> SSLDDKPQFPGASAEFIDKLEFIQPNVISGIPIYRVMDRQGQIINPSEDPHLPKEKVLKLYKSMTLLNTMDRILYESQRQGRISFYMTNYGEEGTHVGSAAALDNTDLVFGQYREAGVLMYRDYPLELFMAQCYGNISDLGKGRQMPVHYGCKERHFVTISSPLATQIPQAVGAAYAAKRANANRVVICYFGEGAASEGDAHAGFNFAATLECPIIFFCRNNGYAISTPTSEQYRGDGIAARGPGYGIMSIRVDGNDVFAVYNATKEARRRAVAENQPFLIEAMTYRIGHHQTSDDSSAYRSVDEVNYWDKQDHPISRLRHYLLSQGWWDEEQEKAWRKQSRRKVMEAFEQAERKPKPNPNLLFSDVYQEMPAQLRKQQESLARHLQTYGEHYPLDHFDK;> VAHFTFQPDPEPREYGQTQKMNLFQSVTSALDNSLAKDPTAVIFGEDVAFGGVFRCTVGLRDKYGKDRVFNTPLCEQGIVGFGIGIAVTGATA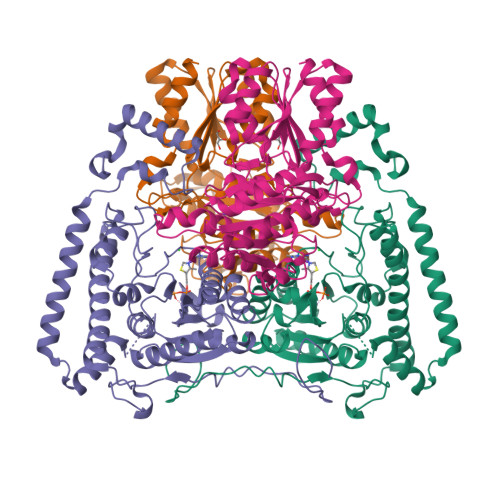IAEIQFADYIFPAFDQIVNEAAKYRYRSGDLFNCGSLTIRSPWGCVGHGALYHSQSPEAFFAHCPGIKVVIPRSPFQAKGLLLSCIEDKNPCIFFEPKILYRAAAEEVPIEPYNIPLSQAEVIQEGSDVTLVAWGTQVHVIREVASMAKEKLGVSCEVIDLRTIIPWDVDTICKSVIKTGRLLISHEAPLTGGFASEISSTVQEECFLNLEAPISRVCGYDTPFPHIFEPFYIPDKWKCYDALRKMINY>[3x]MRYIVALTGGIGSGKST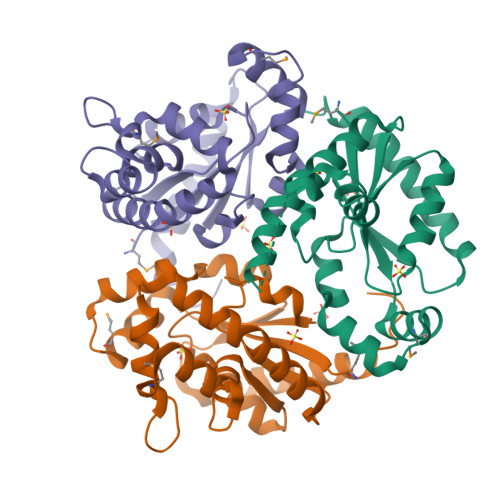VANAFADLGINVIDADIIARQVVEPGAPALHAIADHFGANMIAADGTLQRRALRERIFANPEEKNWLNALLHPLIQQETQHQIQQATSPYVLWVVPLLVENSLYKKANRVLVVDVSPETQLKRTMQRDDVTREHVEQILAAQATREARLAVADDVIDNNGAPDAIASDVARLHAHYLQLASQFVSQEKPGSHHHHHHHH(1S,2R,3S,4R,5S)-5-methyl-7-oxabicyclo[2.2.1]heptane-2,3-dicarboxylic acid | C9 H12 O5 | 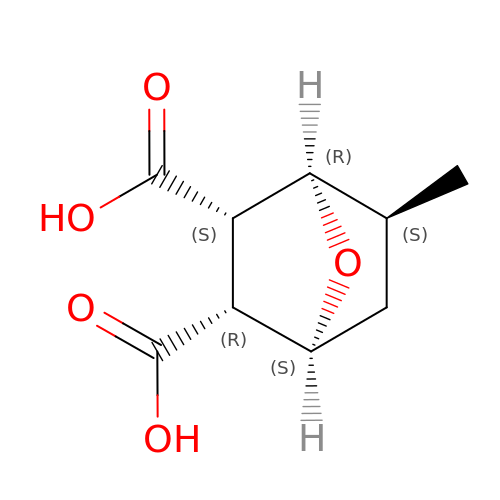YSNMFFYDVUEGJH-AZEWMMITSA-N> MKKLFLVFWWHMHQPLYREPYTGEYLLPWTFFHAVKDYYDMPAYLKDFEIKLNFNLTPVLIDQIQEYAQGKAKDVFLEAIRKDPDDLEKEEVEKLIEFTKLNYEKPIYRFERIRELMNKEKLNREELLDLQTLNLLAWCGRTLRKDLKDLLNKGRNYTQEEKEYVLNKYFEIIKKTLSIYREIKEEGKGSVSTSPYYHPLIPILLNPNCVYETTPNVKIPDFAVSFREDASKHVELAKEKYFEIFGEHPVYMWPPEASVSNEALELYYEKGINMLATDEVILKNSVERASPYLRYYFRELISVFFRDKTLSDLIGFSYHAWNAEDAVRDFIGRLKKIHESVDFQPVVFVVL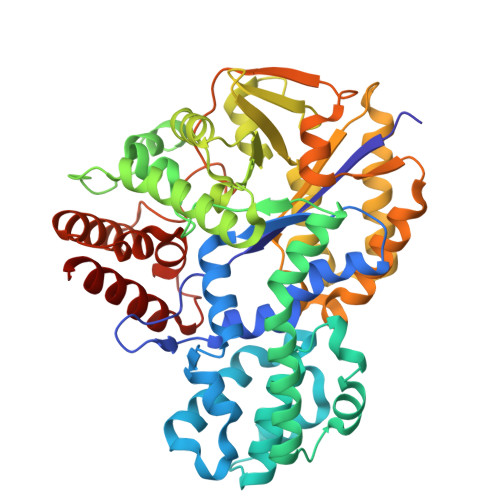DGENCWEYYEENGIPFLEKLYSTLEKEEWIETLTLEEAMRKEDVKTEVIESVKAGTWFDGNFLKWIGNKEKNEYWKILIEAKKKAKNDYILVAEGSDWFWWQGEEKAPFVEVFDKLFRSFVRRAQEH> MEGNKLEEQDSSPPQSTPGLMKGNKREEQGLGPEPAAPQQPTAEEEALIEFHRSYRELFEFFCNNTTIHGAIRLVCSQHNRMKTAFWAVLWLCTFGMMYWQFGLLFGEYFSYPVSLNINLNSDKLVFPAVTICTLNPYRYPEIKEELEELDRITEQTLFDLYKYSSFTTLVAGSRSRRDLRGTLPHPLQRLRVPPPPHGARRAR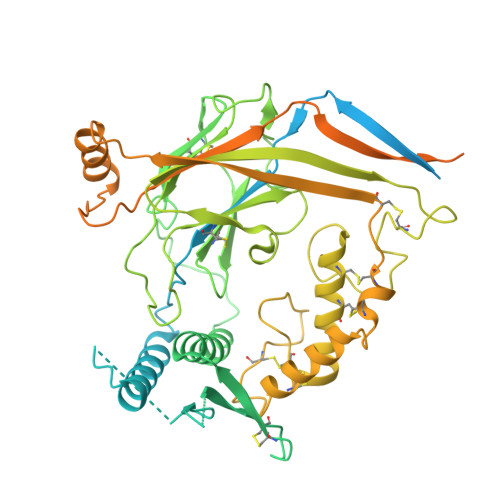SVASSLRDNNPQVDWKDWKIGFQLCNQNKSDCFYQTYSSGVDAVREWYRFHYINILSRLPETLPSLEEDTLGNFIFACRFNQVSCNQANYSHFHHPMYGNCYTFNDKNNSNLWMSSMPGINNGLSLMLRAEQNDFIPLLSTVTGARVMVHGQDEPAFMDDGGFNLRPGVETSISMRKETLDRLGGDYGDCTKNGSDVPVENLYPSKYTQQVCIHSCFQESMIKECGCAYIFYPRPQNVEYCDYRKHSSWGYCYYKLQVDFSSDHLGCFTKCRKPCSVTSYQLSAGYSRWPSVTSQEWVFQMLSRQNNYTVNNKRNGVAKVNIFFKELNYKTNSESPSVTMVTLLSNLGSQWSLWFGSSVLSVVEMAELVFDLLVIMFLMLLRRFRSRYWSPGRGGRGAQEVASTLASSPPSHFCPHPMSLSLSQPGPAPSPALTAPPPAYATLGPRPSPGGSAGASSSTCPLGGP> ELPSLCMLNNSFYYMKGGANIFLIRVSDVSVLMKEYDVSVYEPEDLGNCLNKSDSSWAIHWFSIALGHDWLMDPPMLCRNKTKKEGSNIQFNISKADESRVYGKKIRNGMRHLFRGFYDPCEEGKVCYVTINQCGDPSSFEYCGTNYLSKCQFD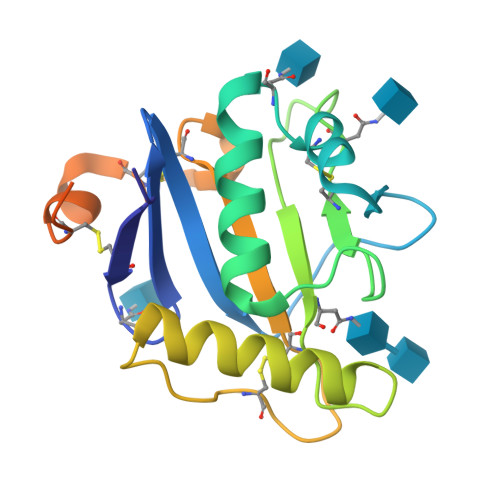HVNTLHFLVRSKTHLNFGTGTKHHHHHH2-(propan-2-yl)-1H-pyrrolo[3,2-b]pyridine | C10 H12 N2 | 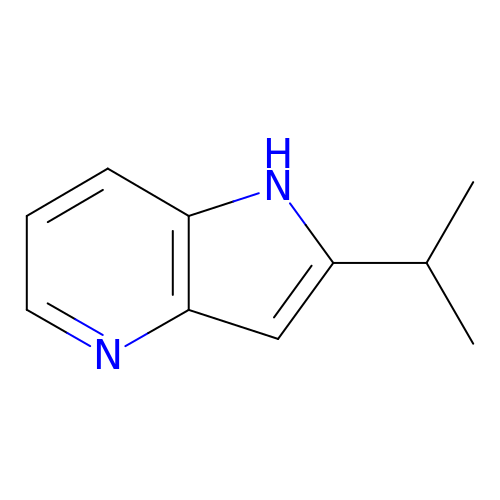OKEHFANNANVSEO-UHFFFAOYSA-N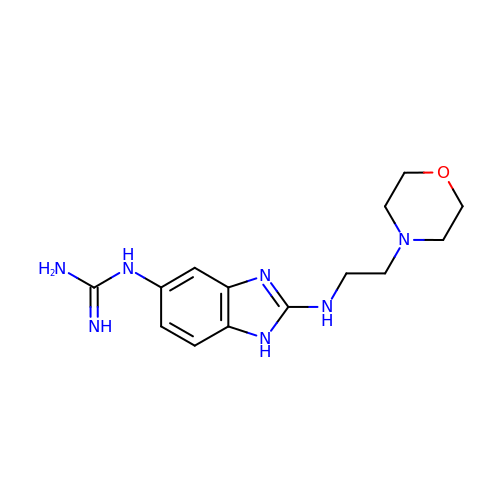N-(2-{[2-(morpholin-4-yl)ethyl]amino}-1H-benzimidazol-5-yl)guanidine | C14 H21 N7 O | GUEKBGQUTZFSQX-UHFFFAOYSA-N> SNAMAMIHKFSMMGTNIVVDVNSGAVHVVDDISFDILDYYKNFTAGEIKNKLAHKYNADEIDEALREIESLEAEGLLFSEDPYKEYVSSMDRKSVVKALCLHISHDCNLRCKYCFASTGNFGGQRNMMSLEVGKKAIDFLISESGNRKNLEIDFFGGEPMMNFDVVKGIIEYARQKEKEHNKNFRFTLTTNGLLLNDENIKYINENMQNIVLSIDGRKEVNDRMRIRIDGSGCYDDILPKFKYVAESRNQDNYYVRGTFTRENMDFSNDVLHLADEGFRQISVEPVVAAK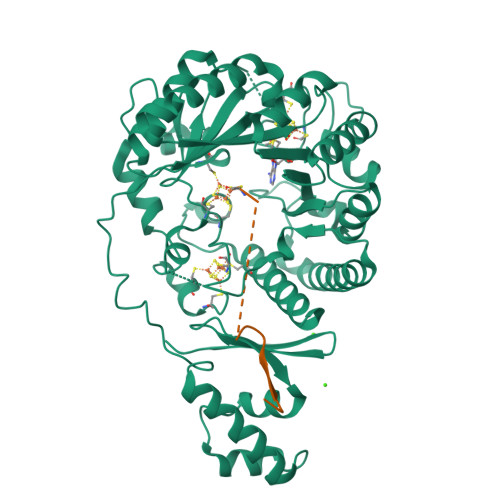DSGYDLREEDLPRLFEEYEKLAYEYVKRRKEGNWFNFFHFMIDLTQGPCIVKRLTGCGSGHEYLAVTPEGDIYPCHQFVGNEKFKMGNVKEGVLNRDIQNYFKNSNVYTKKECDSCWAKFYCSGGCAANSYNFHKDINTVYKVGCELEKKRVECALWIKAQEM;> MKHIKILNGSTLKDSLKKGGC> ERVAVVGVPMDLGANRRGVDMGPSALRYARLLEQLEDLGYTVEDLGDVPVSLARASRRRGRGLAYLEEIRAAALVLKERLAALPEGVFPIVLGGDHSLSMGSVAGAARGRRVGVVWVDAHADFNTPETSPSGNVHGMPLAVLSGLGHPRLTEVFRAVDPKDVVLVGVRSLDPGEKRLLKEAGVRVYTMHEVDRLGVARIAEEVLKHLQGLPLHVSLDADVLD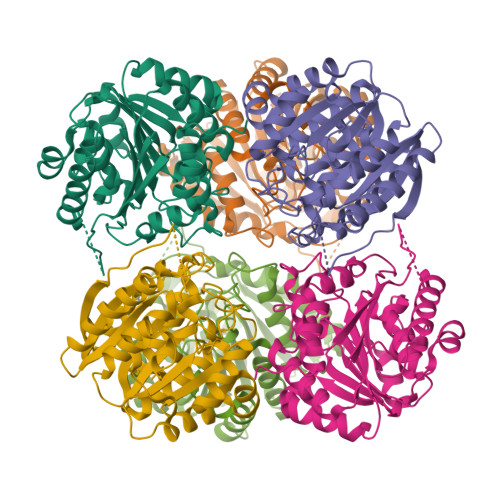PTLAPGVGTPVPGGLTYREAHLLMEILAESGRVQSLDLVEVNPILDERNRTAEMLVGLALSLLGKRIF> SNAMFKEAINNYLHTHGYESIDLKAVLFDMDGVLFDSMPNHAESWHKIMKRFGFGLSREEAYMHEGRTGASTINIVSRRERGHDATEEEIKAIYQAKTEEFNKCPKAERMPGALEVLTKIKSEGLTPMVVTGSGQTSLLDRLNHNFPGIFQANLMVTA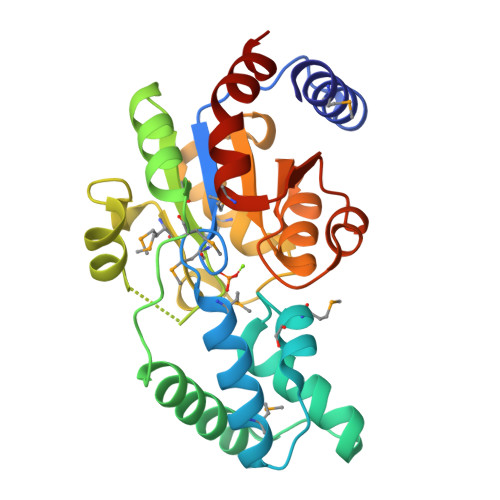FDVKYGKPNPEPYLMALKKGGFKPNEALVIENAPLGVQAGVAAGIFTIAVNTGPLHDNVLLNEGANLLFHSMPDFNKNWETLQSALKQD>CUUGCUGAAGUGCACACAGCAAG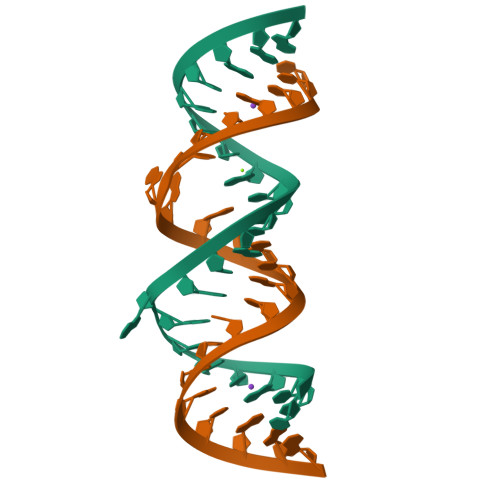[2x]>[2x]MQTVTEPVGSYARAERPQDFEGFVWRLLNDGKEALPRNFRTSADALRAPEKKFHLDAAYVPSREGMDALHISGSSAFTPAQLKNVAAKLREKTAGP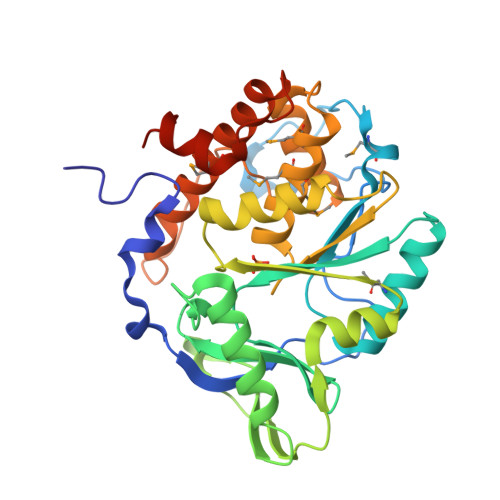IYDVDLSQNSHGYLDGIPVEWYGERNWANLGKSQHEALADERHRLHAALHKTVYIAPLGKHKLPEGGEVRRVQKVQTNQEVAEAAGMRYFRIAATDGVWPTPENIDRFLAFYRTLPQDAWLHFHSHSGVGATTAFMVMTDMLKNPSVSLKDILYRQHEIGGFYYGEFPIKTKDKDSWKTKYYREKIVMIEQFYRYVQENRADGYQTPWSVWLKSHPAKALEHHHHHH> GSHMNDHINLKVAGQDGSVVQFKIKRHTPLSKLMKAYCERQGLSMRQIRFRFDGQPINETDTPAQLEMEDEDTIDVFQQ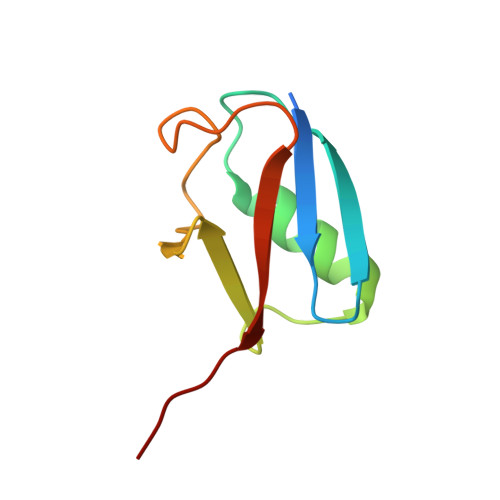QTGG> QDADKLPHTKVTLVAPPQVHPHEQASKTGPKVVEFTMTIEEKKMVIDDKGTTLQAMTFNGSMPGPTLVVHEGDYVQLTLVNPATNAMPHNVDFHGATGALGGAKLTNVNPGEQATLRFKADRSGTFVYHCAPEGMVPWHVVSGQSGTLMVLPRDGLKDPEGKPLHYDRAYTIGEFDLYIPKGPDGKYKDYATLAESYGDTVQVMRTLTPSHIVFNGKVGALTGANALTAKVGETVLLIHSQANRDTRPHLIGGHGDWVWETGKFANPPQRDLETWFIRGGSAGAALYTFKQPGVYAYLNHNLIEAFELGAAGHIKVEGKWNDDLMKQIKAPAPIPR;> QDADKLPHTKVTLVAPPQVHPHEQATKSGPKVVEFTMTIEEKKMVIDDKGTTLQAMTFNGSMPGPTLVVHEGDYVQL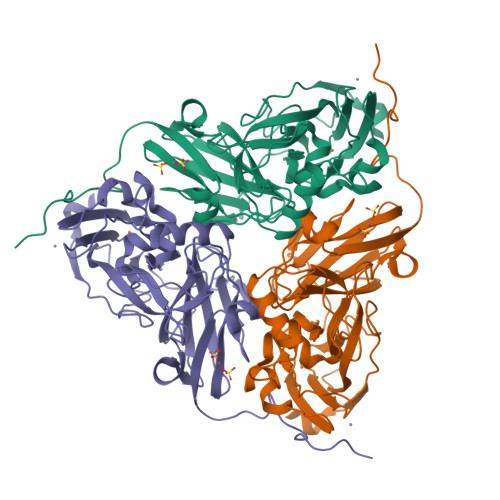TLVNPATNAMPHNVDFHGATGALGGAKLTNVNPGEQATLRFKADRSGTFVYHCAPEGMVPWHVVSGQSGTLMVLPRDGLKDPEGKPLHYDRAYTIGEFDLYIPKGPDGKYKDYATLAESYGDTVQVMRTLTPSHIVFNGKVGALTGANALTAKVGETVLLIHSQANRDTRPHLIGGHGDWVWETGKFANPPQRDLETWFIRGGSAGAALYTFKQPGVYAYLNHNLIEAFELGAAGHIKVEGKWNDDLMKQIKAPAPIPR N-(azidoacetyl)-beta-D-glucopyranosylamine 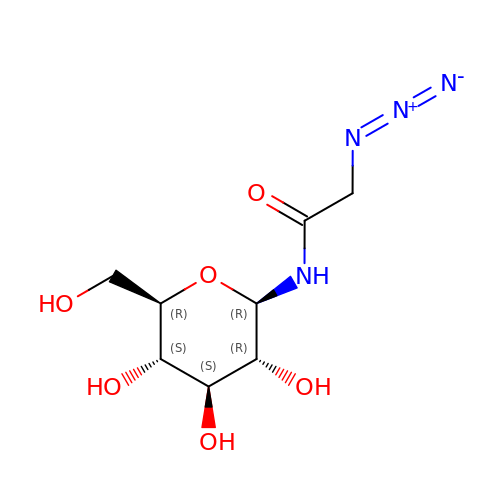| C8 H14 N4 O6 | ACLUEOOMMLAETN-RHROMQPHSA-N> MAYDYKQVLRDSLLFYEAQRSGRLPADQKVTWRKDSALNDQGDQGQDLTGGYFDAGDFVKFGFPMAYTATVLAWGLIDFEAGYSSAGALDDGRKAVKWATDYFIKAHTSQNEFYGQVGQGDADHAFWGRPEDMTMARPAYKIDT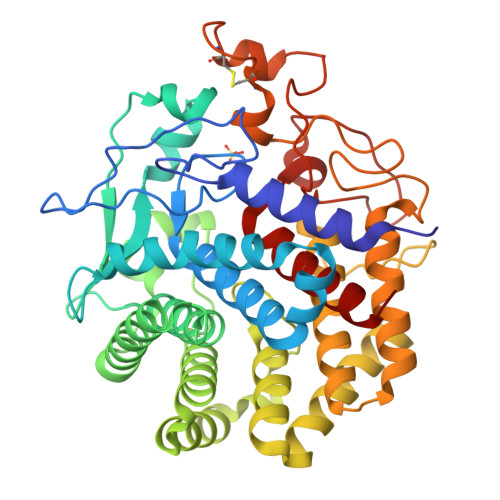SRPGSDLAGETAAALAAASIVFRNVDGTYSNNLLTHARQLFDFANNYRGKYSDSITDARNFYASADYRDELVWAAAWLYRATNDNTYLNTAESLYDEFGLQNWGGGLNWDSKVSGVQVLLAKLTNKQAYKDTVQSYVNYLINNQQKTPKGLLYIDMWGTLRHAANAAFIMLEAAELGLSASSYRQFAQTQIDYALGDGGRSFVCGFGSNPPTRPHHRSSSCPPAPATCDWNTFNSPDPNYHVLSGALVGGPDQNDNYVDDRSDYVHNEVATDYNAGFQSALAALVALGY>[3x]QSMQQLQNVIETAFERRADITPANVDTVTREAITHVIDLLDTGALRVAEKIDGQWVTHQWLKKAVLLSFRINDNQVMEGAETRYYDKVPMKFAGYDEARFQREGFRVVPPATVRKGAFIARNTVLMPSYVNIGAFVDEGTMVDTWATVGSCAQIGKNVHLSGGVGIGGVLEPLQANPTII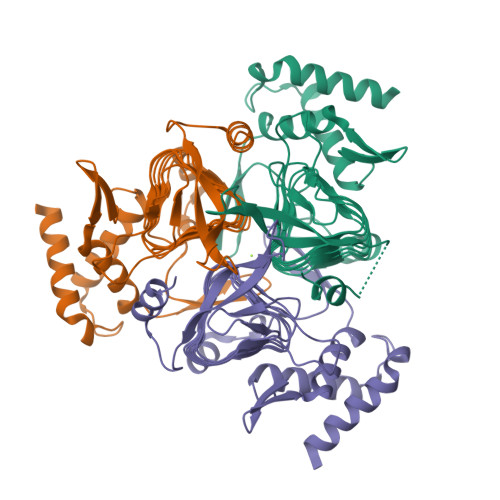EDNCFVGARSEVVEGVIVEEGSVISMGVFIGQSTRIYDRETGEVHYGRVPAGSVVVSGNLPSKDGSYSLYCAVIVKKVDAKTRSKVGINELLRTID1-methyl-6-pyridin-3-yl-pyrazolo[3,4-d]pyrimidin-4-amine 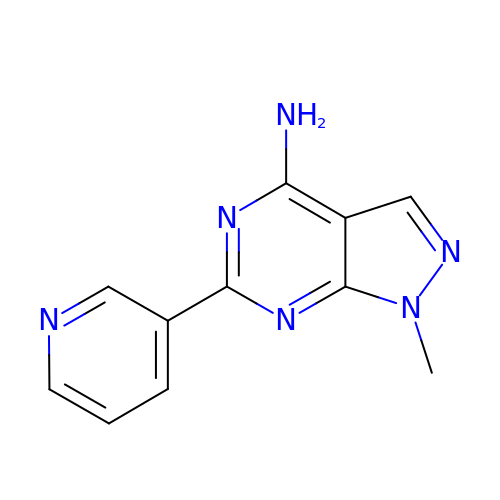| C11 H10 N6 | RWOFPWSZGRSDPB-UHFFFAOYSA-N>GLQGHIIENPQYFSDACVHHIKRRDIVLKWELGEGAFGKVFLAECHNLLPEQDKMLVAVKALKEASESARQDFQREAELLTMLQHQHIVRFFGVCTEGRPLLMVFEYMRHGDLNRFLRSHGPDAKLLAGGEDVAPGPLGLGQLLAVASQVAAGMVYLAGLHFVHRDLATRNCLVGQGLVVKIGDFGMSRDIYSTDYYRVGGRTMLPIRWMPPESILYRKFTTESDVWSFGVVLWEIFTYGKQPWYQLSNTEAIDCITQGRELERPRACPPEVYAIMRGCWQREPQQRHSIKDVHARLQALAQAPPVYLD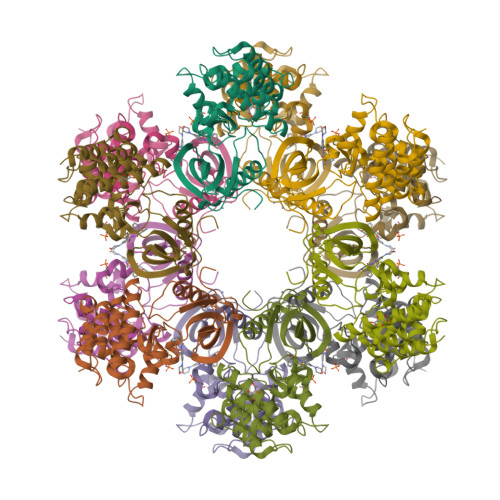VL[3x]>[4x]GHMAPIKVIADKGTPFADLLVPKLTASVTDGAVGVTVDAPVSVTAADGVLAAVTMVNDNGRPVAGRLSPDGLRWSTTEQLGYNRRYTLNATALGLGGAATRQLTFQTSSPAHLTMPYVMPGDGEVVGVGEPVAIRFDENIADRGAAEKAIKITTNPPVEGAFYWLNNREVRWRPEHFWKPGTAVDVAVNTYGVDLGEGMFGEDNVQTHFTIGDEVIATADDNTKILTVR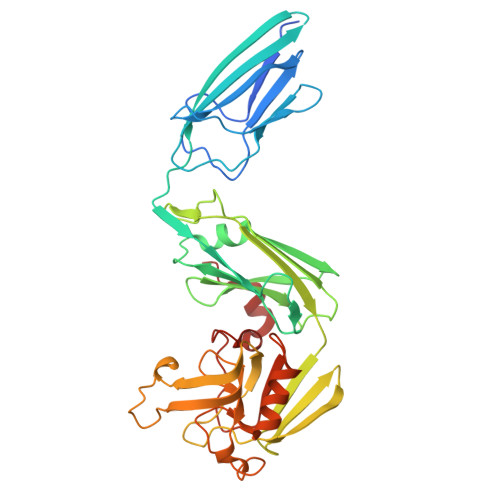VNGEVVKSMPTSMGKDSTPTANGIYIVGSRYKHIIMDSSTYGVPVNSPNGYRTDVDWATQISYSGVFVHSAPWSVGAQGHTNTSHGCLNVSPSNAQWFYDHVKRGDIVEVVNTVGGTLPGIDGLGDWNIPWDQWRAGNAKA> MKLCILLAVVAFVGLSLGRSPWPGVPMSFFSNLRAVNKLYPNQASFITDNTRLLTSTPAGFTNVLNAPSVRNIGNNRFQPGYQLSNNQFVSTSDINRITRNNDVPNIRGVFQGISDPQINSLSQLRRVDNVPDFNYHTKQTRSNAVKQNFPETNVRTPEGVQNALQQNPRLHSYMQSLKVGGTGILLATGGYFLFSAATLVQDIINAINNTGGSYYVQGKDAGEIAEA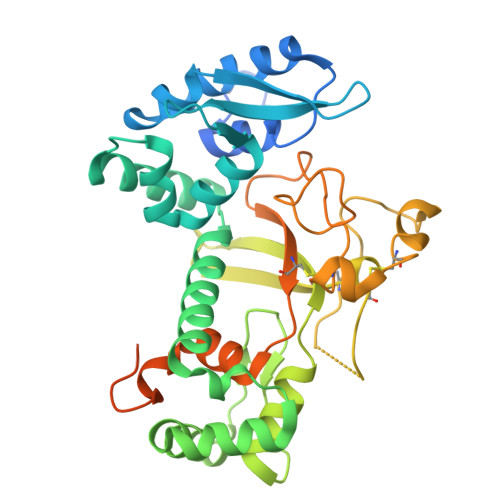CLLLQRTCRQDPNLNQSDVTICPFDPLLPNNPPELTNMCQGFNYEVEKTVCRGSDPSADPDSPQYVDISDLPAGQTLMCIEPYSFGDLVGDLGLDWLLGDEGLVGKSSNVSDSVSGKLMLESRGPFEGKPIPNPLLGLDSTRTGHHHHHH> MTENILRKSDEEIQKEITARVKALESMLIEQGILTTSMIDRMAEIYENEVGPHLGAKVVVKAWTDPEFKKRLLADGTEACKELGIGGLQGEDMMWVENTDEVHHVVVCTLCSCYPWPVLGLPPNWFKEPQYRS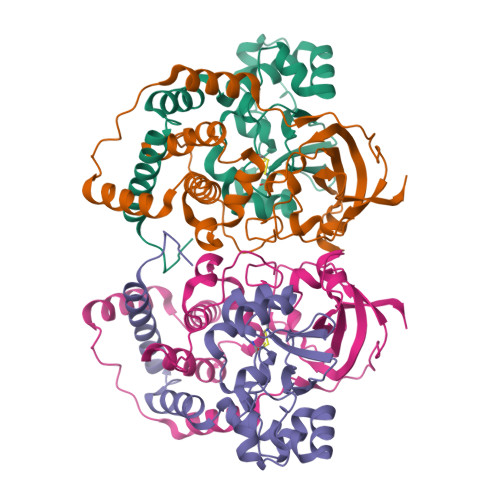RVVREPRQLLKEEFGFEVPPSKEIKVWDASSEMRFVVLPQRPAGTDGWSEEELATLVTRESMIGVEPAKAVAHHHHHH;> MNGVYDVGGTDGLGPINRPADEPVFRAEWEKVAFAMFPATFRAGFMGLDEFRFGIEQMNPAEYLESPYYWHWIRTYIHHGVRTGKIDLEELERRTQYYRENPDAPLPEHEQKPELIEFVNQAVYGGLPASREVDRPPKFKEGDVVRFSTASPKGHARRARYVRGKTGTVVKHHGAYIYPDTAGNGLGECPEHLYTVRFTAQELWGPEGDPNSSVYYDCWEPYIELVDTKAAAA> MIVSSSIVFDIFNYIGIVAFAISGAIKAVKKGMDLLGVLVLGFSTALGGGIISNLLLGKTPPTNLIYYPYPITAFLASLATFVFYRIFTNVGKPLLYADAIGLGAFASSGASLAYSVSNNVILVVIVGAITAVGGGVIRDILSNEVPLILTREFYATTAVIGSFVYFIASDLSVPEDVALIVSFLITLILRILAMELKWELPRKKIEAAAENLYFQGLEDYKDDDDKHHHHHHHHHH

As evidenced by the fact that their genetic ablation led to compromised K+ permeability and Ca2+ release across the SR/ER membrane, TRICs play important roles as counter-ion channels for balancing the charge potential change during Ca2+ release/uptake in the intracellular stores. In this study, we analyse the structure and function of a bacterial and an archaeal TRIC channel. Both proteins have similar structures, consisting in symmetric trimers of 7-TM subunits, each composed as inverted quasi-repeats of triple-helix bundles (THBs) plus an added TM segment (TM7). Many other trimeric channels, including ATP-gated P2X receptors, acid-sensing ion channels40 and the mechanosensitive Piezo1 channels41, form central ion-conducting pores at the three-fold axes of protomer association; by contrast, the prokaryotic TRIC trimers have three pores as calculated by the HOLE programme, one through each protomer.

The structure for the wild-type protein in another lattice was solved by molecular replacement and extended to 1.6 Å resolution (type 2a, in P63 lattice). The final model for SaTRIC was refined to Rwork/Rfree values of 16.8%/17.9%, containing ordered residues 7–200, two Na+ ions and 90 water molecules. In the SaTRIC structure at 1.6 Å resolution, an intriguing set of nine electron density features occupies each pore. We identified these densities as water molecules on the basis of their coordination with the surrounding residues. The cytoplasmic closure of the pore is due to a hydrogen-bonded network of interactions among C-THB residues D99 (TM4)–R139-D140 (TM5)–Y155 (TM6). We describe this arrangement as a ‘locked' conformation of C-THB. By contrast, interactions among the quasi-symmetric mates in N-THB, N13 (TM1)–S53-N54 (TM2)–Y70 (TM3), are mostly undone; thereby, N-THB is released to an unlocked, pore-open conformation. This asymmetry in the inverted pair of THBs, with C-THB in a locked state versus N-THB in an unlocked state, generates an open-outward conformation. The high-resolution structure clearly reveals that these glycine motifs generate similar kinks (∼41° in TM2 and ∼45° in TM5) near the middle of the respective TM segments, disrupting the normal α-helical hydrogen-bonding pattern and exposing backbone amines that coordinate bridging water molecules. Two monovalent Na+ ions, each with three bound water molecules, were bound in the 1.6 Å-resolution type 2a structure, while in the 1.9 Å-resolution type 2b structure, obtained from a different condition, a single divalent Mg2+ ion was bound at the same site, with slight adjustment on the N144 side chain and also with three bound water molecules. The well-defined series of water molecules through each protomer of the high-resolution type 2a SaTRIC structure and sensitivity of conduction properties to mutations of associated residues define a putative ion conduction pathway.> SHDSLRPKLSEEQQHIIAILLDAHHKTYDPTYADFRDFRPPVRMDGSTGSVTLDLSPLSMLPHLADLVSYSIQKVIGFAKMIPGFRDLTSDDQIVLLKSSAIEVIMLRSNQSFTMDDMSWDCGSQDYKYDVTDVSKAGHTLELIEPLIKFQVGLKKLNLHEEEHVLLMAICIVSP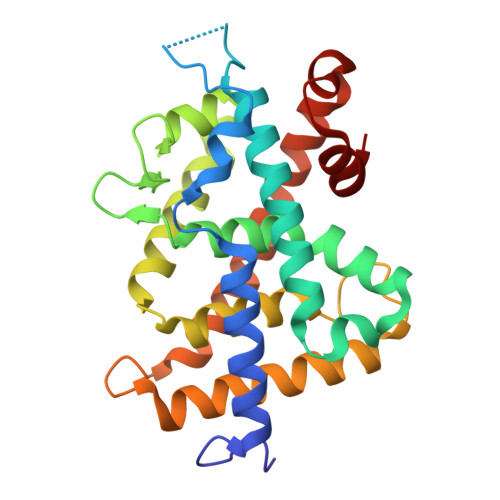DRPGVQDAKLVEAIQDRLSNTLQTYIRCRHPPPGSHQLYAKMIQKLADLRSLNEEHSKQYRSLSFQPENSMKLTPLVLEVFGN> MVPISPIETVPVKLKPGMDGPKVKQWPLTEEKIKALVEICTEMEKEGKISKIGPENPYN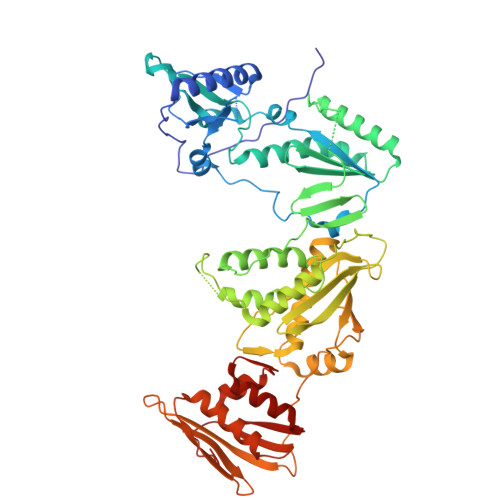TPVFAIKKKWRKLVDFRELNKRTQDFWEVQLGIPHPAGLKKKKSVTVLDVGDAYFSVPLDEDFRKYTAFTIPSINNETPGIRYQYNVLPQGWKGSPAIFQSSMTKILEPFAAQNPDIVIYQYMDDLYVGSDLEIGQHRTKIEELRQHLLRWGLTTPAKEPPFLWMGYELHPDKWTVQPIVLPEKDSWTVNDIQKLVGKLNWASQIYPGIKVRQLSKLLRKALTEVIPLTEEAELELAENREILKEPVHGVYYDPSKDLIAEIQKQGQGQWTYQIYQEPFKNLKTGKYARMRGAHTNDVKQLTEAVQKITTESIVIWGKTPKFKLPIQKETWETWWTEYWQATWIPEWEFVNTPPLVKLWYQLEKEPIVGAETFYVDGAANRETKLGKAGYVTNKGRQKVVPLTNTTNQKTELQAIYLALQDSGLEVNIVTDSQYALGIIQAQPDKSESELVNQIIEQLIKKEKVYLAWVPAHKGIGGN>[2x]MAREFSLEKTRNIGIIAHIDAGKTTTTERILYYTGRIHKIGETHEGASQMDWMEQEQDRGITITSAATTAAWEGHRVNIIDTPGHVDF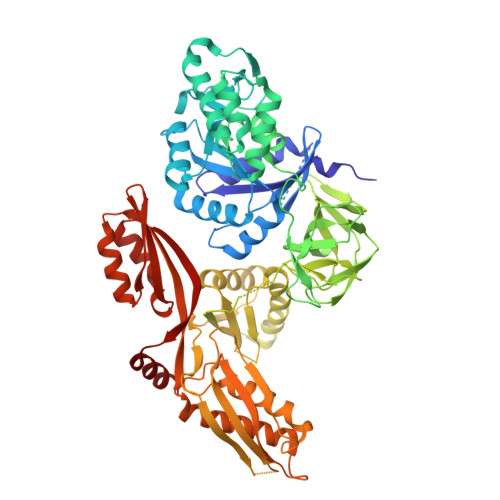TVEVERSLRVLDGAVTVLDAQSGVEPQTETVWRQATTYGVPRIVFVNKMDKLGANFEYSVSTLHDRLQANAAPIQLPIGAEDEFEAIIDLVEMKCFKYTNDLGTEIEEIEIPEDHLDRAEEARASLIEAVAETSDELMEKYLGDEEISVSELKEAIRQATTNVEFYPVLCGTAFKNKGVQLMLDAVIDYLPSPLDVKPIIGHRASNPEEEVIAKADDSAEFAALAFKVMTDPYVGKLTFFRVYSGTMTSGSYVKNSTKGKRERVGRLLQMHANSRQEIDTVYSGDIAAAVGLKDTGTGDTLCGEKNDIILESMEFPEPVIHLSVEPKSKADQDKMTQALVKLQEEDPTFHAHTDEETGQVIIGGMGELHLDILVDRMKKEFNVECNVGAPMVSYRETFKSSAQVQGKFSRQSGGRGQYGDVHIEFTPNETGAGFEFENAIVGGVVPREYIPSVEAGLKDAMENGVLAGYPLIDVKAKLYDGSYHDVDSSEMAFKIAASLALKEAAKKCDPVILEPMMKVTIEMPEEYMGDIMGDVTSRRGRVDGMEPRGNAQVVNAYVPLSEMFGYATSLRSNTQGRGTYTMYFDHYAEVPKSIAEDIIKKNKGE> GLFDAPGRS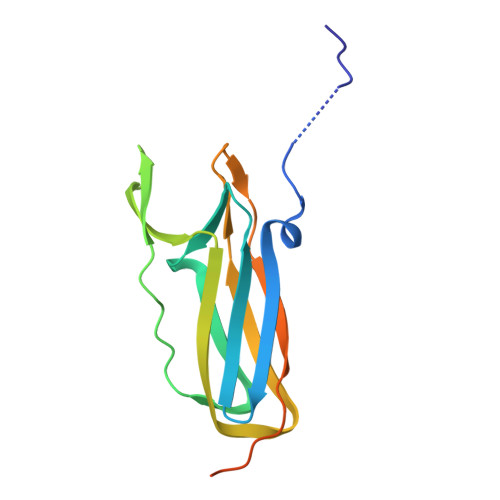QFVPADQAFAFDFQQNQHDLNLTWQIKDGYYLYRKQIRITPEHAKIADVQLPQGVWHEDEFYGKSEIYRDRLTLPVTINQASAGATLTVTYQGSADAGFCYPPETKTVPLSEVVANNAAPQPVSVPQQEQPTAQ>[2x]GPGSHLAHPNLDTFTPEELLQQMKELLTKNHQLKEAMKLNNQAMKGRFEELSAWTEKQKEERQFFEIQSKEAKERLMALSHE;>GPGSYPSSNTLVEMTLGMKKLKEEMEGVVKELAENNHILERFGSLTMDGGLRNVDCL[2x]

OPTN is an ubiquitin-binding autophagy receptor, which is initially found to participate in the xenophagy and aggrephagy processes, and more recently is also demonstrated to involve in the PARKIN-dependent mitophagy. The N-terminal coiled-coil region of OPTN is responsible for its interaction with TANK-binding kinase 1 (TBK1), which is a noncanonical IκB kinase family member involved in innate immunity and autophagy. Here we biochemically and structurally characterize the interaction between OPTN and TBK1, and demonstrate that the direct association of OPTN N-terminal coiled-coil domain (NTD) with TBK1 CTD domain is responsible for the OPTN/TBK1 complex formation. The structures of OPTN NTD in complex with TBK1 CTD and the related NAP1/TBK1 complex solved in this study not only elucidate the detailed molecular mechanism underlying the OPTN and TBK1 interaction but also uncover a general interaction mode governing TBK1's binding to all of its currently identified binding adaptor proteins.

Among the OPTN mutations, the glaucoma-associated E50K mutation is demonstrated to associate with a more progressive and severe disease phenotype, and causes death of retinal ganglion cells in transgenic mice. Obviously, the E50K mutation would disrupt the salt bridge interaction seen in the wild-type OPTN/TBK1 complex, but, surprisingly, the OPTN E50K mutant shows a roughly 43-fold increase of binding affinity towards TBK1 compared with the wild-type protein, consistent with our Co-IP result and several earlier observations that the E50K mutation would increase the interaction between OPTN and TBK1 in cells. To further elucidate the detailed mechanism, we also solved the structure of OPTN(26–103) E50K mutant in complex with TBK1 CTD. To our surprise, the overall structure of the mutant complex is almost the same as that of the OPTN(26–103)/TBK1(677–729) complex. However, detailed structural analysis revealed that the positively charged OPTN K50 residue in the mutant complex forms a charge–charge interaction with the negatively charged TBK1 E698 residue, and meanwhile its long aliphatic side chain packs extensively with the hydrophobic pocket formed by the side chain of OPTN L47 and TBK1 M697 residues. Given that the OPTN/TBK1 complex is a symmetrical tetramer, these additional synergic interactions induced by the E50K mutation likely contribute to the increase of binding affinity observed between OPTN E50K mutant and TBK1. Interestingly, multi-angle light scattering (MALS) analysis revealed that the E50K mutation could change the oligomeric state of OPTN N-terminal region (residues 1–119) and induce its tetramerization. Collectively, these data demonstrated that the POAG-associated OPTN E50K mutation not only enhances the interaction between OPTN and TBK1 but also affects the oligomeric state of OPTN.> GHMASSENASSAKLSVPERQKLAQQSAGKVLTLLDLSEVQLDGAATLVLTFSIPLDPDQDFSRVIHVVDKKSGKVDGAWELSDNLKEL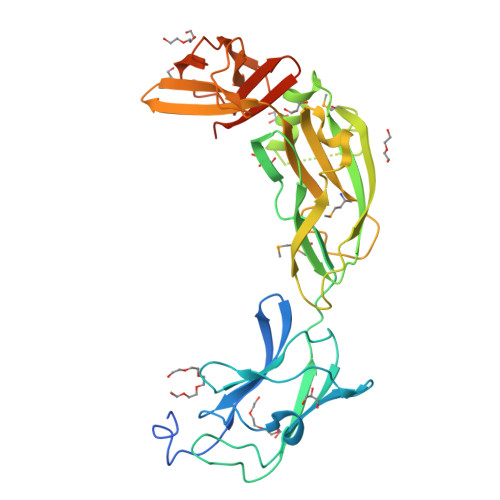RLRHLEPKRDLIVTIGKEVKALNNATFSKDYEKTITTRDIQPSVGFASRGSLLPGKVVEGLPVMALNVNNVDVNFFRVKPESLPAFISQWEYRNSLANWQSDKLLQMADLVYTGRFDLNPARNTREKLLLPLGDIKPLQQAGVYLAVMNQAGRYDYSNPATLFTLSDIGVSAHRYHNRLDIFTQSLENGAAQQGIEVSLLNEKGQTLTQATSDAQGHVQLENDKNAALLLARKDGQTTLLDLKLPALDLAEFNIAGAPGYS>[16x]MHHHHHHMKSIDEQSLHNARRLFESGDIDRIEVGTTAGLQQIHRYLFGGLYDFAGQIREDNISKGGFRFANAMYLKEALVKIEQ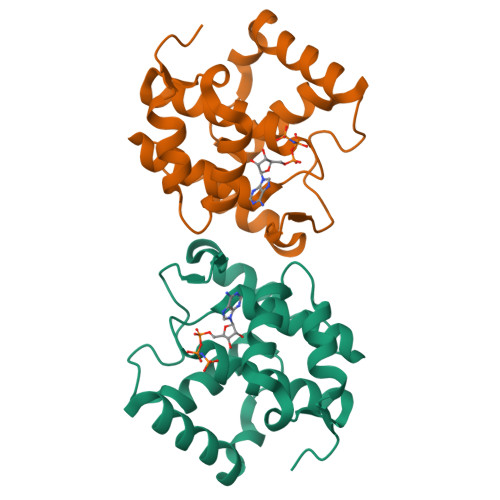MPERTFEEIIAKYVEMNIAHPFLEGNGRSTRIWLDLVLKKNLKKVVNWQNVSKTLYLQAMERSPVNDLELRFLLKDNLTDDVDNREIIFKGIEQAYYYAGYEKG>[2x]MVKLMEVYEGKAKKMIPIDDDKLIMEFKDDATAFDGTKKARFKGKGWLNAQLS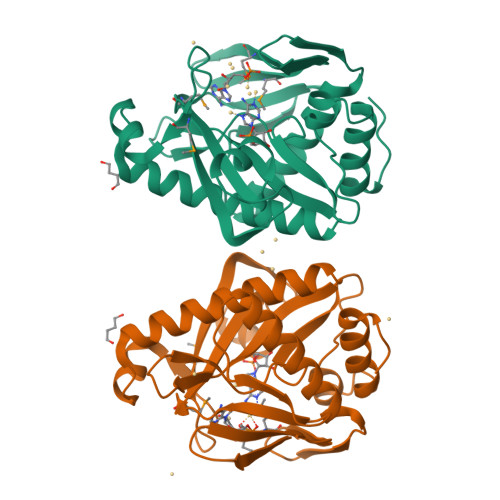VIFFKLLEEHGIKTHFIGVAGGNRLIVEKLDMYPLEVVVRNVVAGSLKKRLPLPEGYELPEPIVELYYKNDELHDPMINYYHAKVLGISLDEIKKIEEIALKVNEILKDYLAKKGIILVDFKLEFGKDKNGDIVLADEISPDTCRFWDAKTKRSLDKDVFRFDKGDLIEAYKEIYERITGEKPEF Ziprasidone | C21 H21 Cl N4 O S | 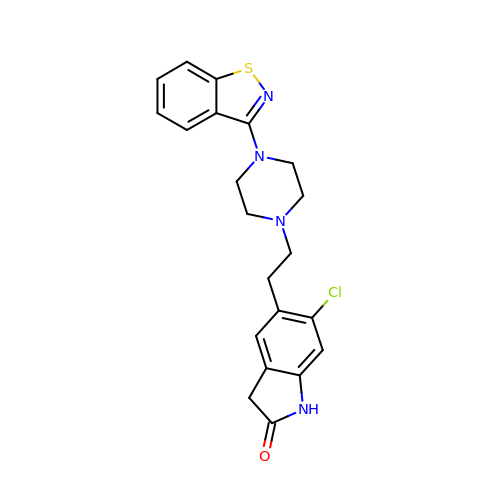MVWVFYHBGMAFLY-UHFFFAOYSA-N> MSSTMKDTQEAPVRWSRNWTPDAIRALVDQDNGKLDARIYADQDLYQLELERVFGRSWLMLGHETHIPKIGDYLTTYMGEDPVIMVRQKDQSIKVFLNQCRHRGMRIVRSDGGNAKAFTCTYHGWAYDIAGNLVNVPFEKEAFCDKKEGDCGFDKADWGPLQARVETYKGLVFANWDPEAPDLKTYLSDAMPYMDVMLDRTEAGTEAIGGIQKWVIPCNWKFAAEQFCSDMYHAGTMSHLSGVLAGLPPEMDLTQIQLSKNGNQFRSAWGGHGAGWFINDSSILLSVVGPKITQYWTQGPAAEKAARRVPQLPILDMFGQHMTVFPTCSFLPGINTIRTWHPRGPNEVEVWAFVLVDADAPEDIKEEFRLQNIRTFNAGGVFEQDDGENWVEIQRVMRGHKAKSTSLCAKMGLNVPNKNNPAYPGKTAYVYAEEAARGMYHHWSRMMSEPSWDTLKP;> MISTPLSKEFEWPAKPVSLELQHQVEQFYYREAQLLDHHAFQAWFALLAEDIHYWMPIRTVRTAREQGLEYVPAGANAHFDDTHATMYGRIRQKTSDLNWAEDPPSRTRHLVSNVIVREMDTPGTLEVASAFLLYRSRLERQVDVFAGERRDVLRIADNPLGFQIAKRTIILDQSTVLANNLSVFF

Biphenyl dioxygenase is the first enzyme of the Bph pathway and the major determinant of PCB degradation. The catalytic component of this enzyme is a Rieske-type oxygenase (RO), which catalyzes the highly regio- and stereoselective insertion of dioxygen into an aromatic ring, activating the latter for subsequent catabolism. BPDOB356 is a typical heterohexameric RO with αβ protomers arranged about a three-fold symmetry axis to place the Rieske Fe2S2 cluster of each α-subunit within ∼12 Å of the mononuclear Fe(II) of an adjacent α-subunit. Structure of the α-Subunit - The α-subunit of BPDOB356 has two domains: a smaller Rieske ferredoxin domain and a larger mononuclear Fe(II)-containing catalytic domain, in agreement with other characterized ROs.

Here we present the crystal structures of BPDOB356 at 1.6 Å resolution, and BPDOB356 in complex with its substrate biphenyl at 1.6 Å resolution. The coordination sphere of the mononuclear iron is remarkably similar in the BPDOB356:biphenyl complex. As in the substrate-free enzyme, the iron is pentacoordinate and of square pyramidal geometry. H239 is the axial ligand, and the Fe is displaced toward it out of the basal plane by 0.5 Å. In the BPDOB356•biphenyl complex, the 2,3-carbons are 4.3 Å from the Fe(II) and the dihedral angle between the two aromatic rings is 112°. However, the adjustments in protein conformation that accompany binding of biphenyl are much less dramatic in BPDOB356 than in BPDORHA1. In particular, upon binding of biphenyl to BPDOB356, the side chain torsion angles of I283 in the D subsite adjust slightly to move the Cδ1 atom away from biphenyl. The structure of BPDOB356 may illuminate active site structural factors required for potent PCB-degrading ROs in Group I. Although binding of biphenyl to BPDOB356 required only minor adjustments by the protein, biphenyl binding to BPDORHA1 required extensive conformational changes that expand the active site. M231α was chosen because of its unique location at the junction of the P and D subsites and the placement of the M231 Sδ atom in the plane of the proximal ring of biphenyl and near an ortho carbon atom on that ring. Substitution of a chlorine at this ortho carbon position would result in a stearic clash with the M231 Sδ atom.>GSFTMADLDDIKDGKDFRTDQPQKNIPFTLKGCGALDWGMQSRLSRIFNPKTGKTVMLAFDHGYFQGPTTGLERIDINIAPLFEHADVLMCTRGILRSVVPPATNRPVVLRASGANSILAELSNEAVALSMDDAVRLNSCAVAAQVYIGSEYEHQSIKNIIQLVDAGMKVGMPTMAVTGVGKDMVRDQRYFSLATRIAAEMGAQIIKTYYVEKGFERIVAGCPVPIVIAGGKKLPEREALEMCWQAIDQGASGVDMGRNIFQSDH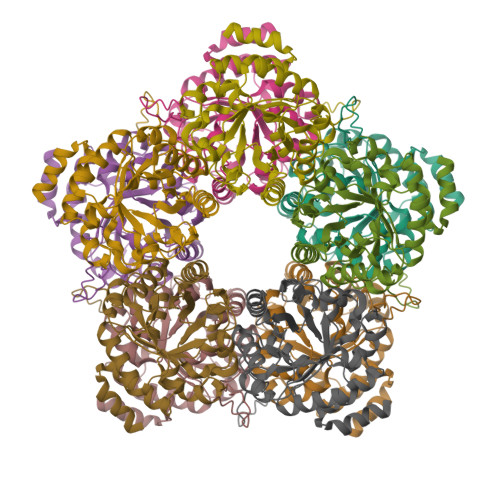PVAMMKAVQAVVHHNETADRAYELYLSEKQ[20x]>[4x]SHMTPKELLEWQTNWKKIMKRDSRIYFDITDDVEMNTYNKSKMDKRRDLLKRGFLTLGAQITQFFDTTVTIVITRRSVENIYLLKDTDILSRAKKNYMKVWSYEKAARFLKNLDVDLDHVDSGASGGSKFSQEQIGENIVCRVICTTGQIPIRDLSADISQVLKEKRSIKKVWTFGRNPACDYHLGNISRLSNKHFQILLGEDGNLLLNDISTNGTWLNGQKVEKNSNQLLSQGDE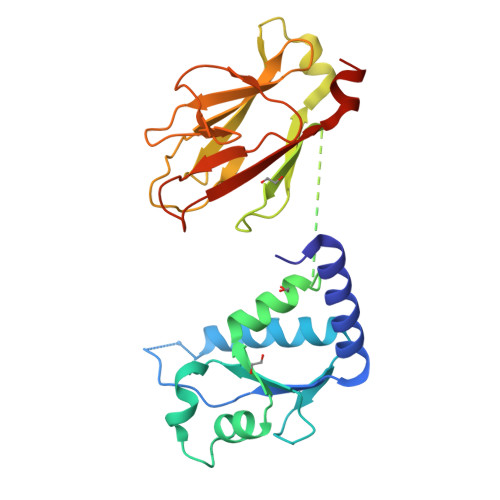ITVGVGVESDILSLVIFINDKFKQCLEQNKVDR In this study, we report the crystal structures of three forms of Tk-PTP, which showed that this protein forms a canonical DUSP fold and that it undergoes an atypical temperature-dependent conformational change between two forms. Structural and biochemical analyses revealed that this structural alteration requires the presence of the GG motif in the P-loop, and that Tk-PTP has dual amino acids, Asp63 and Glu132, both functioning as the general acid/base residues. PTP proteins commonly share a highly conserved active site motif called the PTP signature motif, which is also present in Tk-PTP as HC93MGGLGR99. This motif, constituting the phosphate binding loop (or simply called P-loop), contains the catalytic cysteine residue (Cys93) that functions as a nucleophile for dephosphorylation and the conserved arginine residue (Arg99) that anchors the phosphate group of the substrate during the enzyme reaction.

To confirm whether the unusual structural conversion of Tk-PTP is indeed associated with the presence of a flexible GG motif within its P-loop, we prepared a recombinant Tk-PTP protein containing the Gly95Ala mutation, referred to as Tk-PTP(G95A). The GG motif within the Tk-PTP P-loop was abolished by this mutation; therefore, it was expected that Tk-PTP(G95A) would have a canonically arranged P-loop, similar to that of Tk-PTP(form II). Tk-PTP(G95A) was expressed and purified as was Tk-PTP(form I), and then subjected to crystallization trials without being heated. The structure of Tk-PTP(G95A) was determined up to a resolution of 2.3 Å using cubic-shaped crystals with the space group H3. Intriguingly, the resulting crystal structure of Tk-PTP(G95A) was nearly identical to that of Tk-PTP(form II), especially in terms of the conformation of both P-loop and α4−α5 loop. The P-loop of Tk-PTP(G95A) matched very well with that of Tk-PTP(form II) with RMSDs of 0.16 Å over eight Cα atoms and 0.25 Å over the entire 55 atoms. Accordingly, the ϕ and ψ dihedral angles of the 4th (Ala95) and 5th (Gly96) residues of the Tk-PTP(G95A) P-loop are similar to those of Tk-PTP(form II), but quite different from those of Tk-PTP(form I). Taken together, the α4−α5 loop of Tk-PTP(G95A) is structurally similar to the corresponding loop of Tk-PTP(form II). Collectively, this structural analysis indicates that Tk-PTP(G95A) adopts an enzymatically active structure even without heat treatment, and that the presence of the unusual GG motif in the P-loop enables the described structural flexibility of wild-type Tk-PTP, the characterizing feature of this protein differentiating it from other PTP proteins. The catalytic activities of Tk-PTP(G95A), which constitutively adopts a catalytically active form, was also measured by the same method.

>[3x]MWPSAKFIDGRVAFSRMPAERELDEVARDFDAVVVLVEDYELPYSLDEWEKRGVEVLHGPIPDFTAPSVEQLLEILRWIEERVREGKKVLIHCMAGLGRSGTVGVAWLMYSRGLSLREALMEVRRKRPGAVETQEQMEVLKELEERIKLAAALEHHHHHH>PSVYDAAAQLTADVKKDLRDSWKVIGSDKKGNGVALMTTLFADNQETIGYFKRLGNVSQGMANDKLRGHSI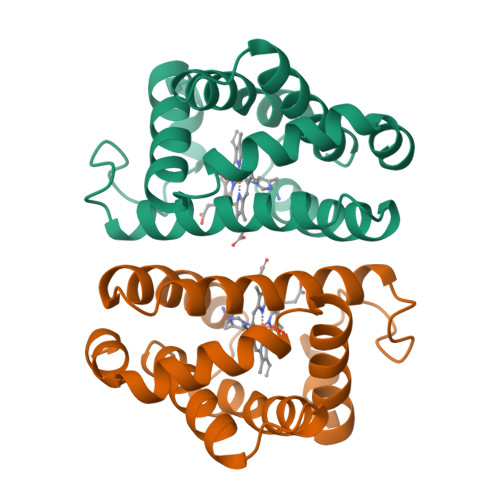TLMYALQNFIDQLDNPDDLVCVVEKFAVNHITRKISAAEFGKINGPIKKVLASKNFGDKYANAWAKLVAVVQAAL[2x]> MGHLPQMGYDRAITVFSPDGRLFQVEYAREAVKRGATAIGIKCKEGVILIADKRVGSKLLEADTIEKIYKIDEHICAATSGLVADARVLIDRARIEAQINRLTYDEPITVKELAKKICDFKQQY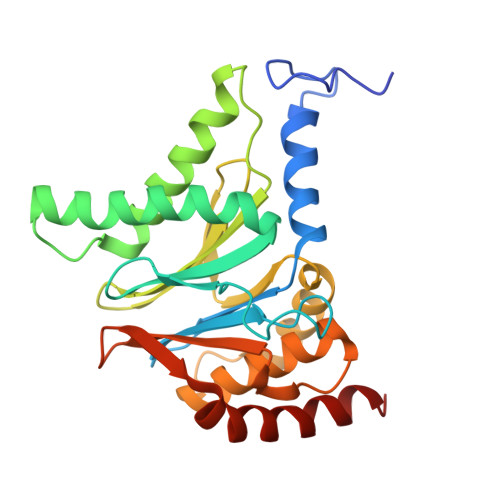TQYGGVRPFGVSLLIAGVDEVPKLYETDPSGALLEYKATAIGMGRNAVTEFFEKEYRDDLSFDDAMVLGLVAMGLSIESELVPENIEVGYVKVDDRTFKEVSPEELKPYVERANERIRELLKK> SPNVEACGYSDRVRQITLGNSTITTQEAANAIVAYGEWPTYINDSEANPVDAPTEPDVSSNRFYTLESVSWKTTSRGWWWKLPDCLKDMGMFGQNMYYHYLGRSG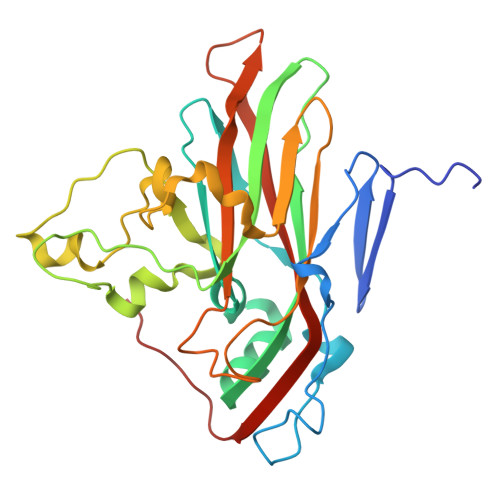YTIHVQCNASKFHQGALGVFLIPEFVMACNTESKTSYVSYINANPGERGGEFTNTYNPSNTDASEGRKFAALDYLLGSGVLAGNAFVYPHQIINLRTNNSATIVVPYVNSLVIDCMAKHNNWGIVILPLAPLAFAATSSPQVPITVTIAPMCTEFNGLRNITVPVHQ1,4-DIPHENYL-2-BUTENE | C16 H16 | 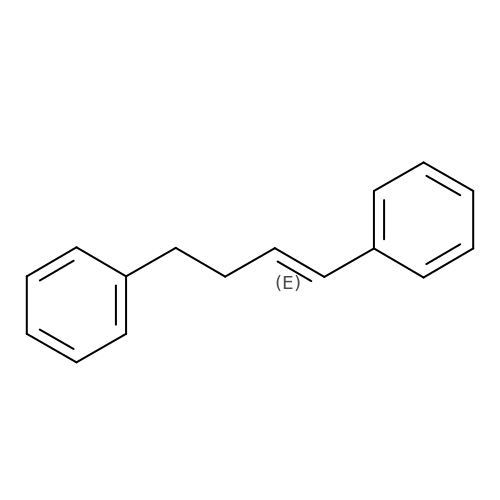NJJOGKAVAWZLAU-NTUHNPAUSA-N>MHHHHHHHHGS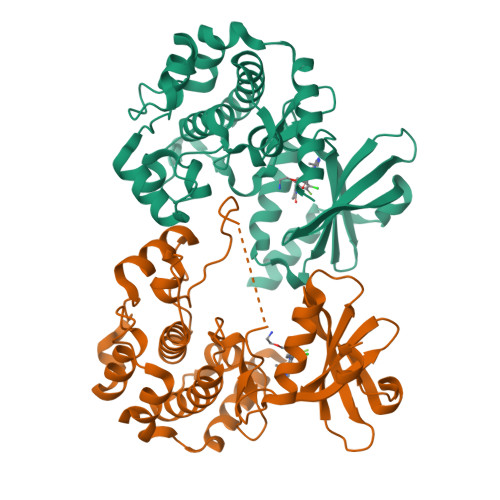PILGYWKIKGLVQPTRLLLEYLEEKYEEHLYERDEGDKWRNKKFELGLEFPNLPYYIDGDVKLTQSMAIIRYIADKHNMLGGCPKERAEISMLEGAVLDIRYGVSRIAYSKDFETLKVDFLSKLPEMLKMFKDRLCHKTYLNGDHVTHPDFMLYDALDVVLYMDPMCLDAFPKLVCFKKRIEAIPQIDKYLKSSKYIAWPLQGWQATFGGGDHPPKSDGENLYFQGSDEEILEKLRSIVSVGDPKKKYTRFEKIGQGASGTVYTAMDVATGQEVAIKQMNLQQQPKKELIINEILVMRENKNPNIVNYLDSYLVGDELWVVMEYLAGGSLTDVVTETCMDEGQIAAVCRECLQALEFLHSNQVIHRNIKSDNILLGMDGSVKLTDFGFCAQITPEQSKRSEMVGTPYWMAPEVVTRKAYGPKVDIWSLGIMAIEMIEGEPPYLNENPLRALYLIATNGTPELQNPEKLSAIFRDFLNRCLEMDVEKRGSAKELLQHQFLKIAKPLSSLTPLIAAAKEATKNNHGNS[2x]> MTKQYLTHRCLIAPPEMADDFFANTVIYLARHDEEGAQGIIINRPAGIQIKELLNDLDIDADNVNPHEVLQGGPLRP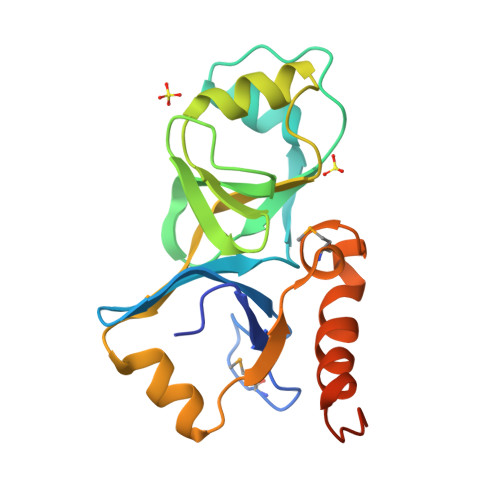EAGFVLHTGQPTWHSSIAVGENVCITTSKDILDAIAHNEGVGRYQIALGYASWGKNQLEDEIARGDWLICDADMDLIFNLPYDDRWDAAYKKIGVDRTWLASEIGHALEHHHHHH> AATPAAVTCQLSNWSEWTDCFPCQDKKYRHRSLLQPNKFGGTICSGDIWDQASCSSSTTCVRQAQCGQDFQCKETGRCLKRHLVCNGDQDCLDGSDEDDCEDVRAIDEDCSQYEPIPGSQKAALGYNILT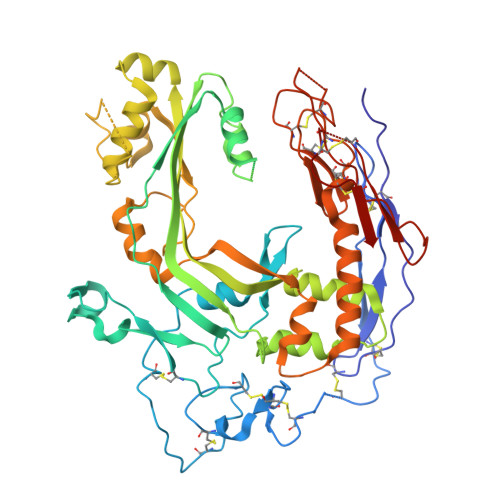QEDAQSVYDASYYGGQCETVYNGEWRELRYDSTCERLYYGDDEKYFRKPYNFLKYHFEALADTGISSEFYDNANDLLSKVKKDKSDSFGVTIGIGPAGSPLLVGVGVSHSQDTSFLNELNKYNEKKFIFTRIFTKVQTAHFKMRKDDIMLDEGMLQSLMELPDQYNYGMYAKFINDYGTHYITSGSMGGIYEYILVIDKAKMESLGITSRDITTCFGGSLGIQYEDKINVGGGLSGDHCKKFGGGKTERARKAMAVEDIISRVRGGSSGWSGGLAQNRSTITYRSWGRSLKYNPVVIDFEMQPIHEVLRHTSLGPLEAKRQNLRRALDQYLMEFNACRCGPCFNNGVPILEGTSCRCQCRLGSLGAACEQTQTEGAKADGSWSCWSSWSVCRAGIQERRRECDNPAPQNGGASCPGRKVQTQAC>MFIKAERLLIRKFEFKDWEAVHEYTSDSDVMKYIPEGVFTEEDTRNFVNKNMGENAKNFPVILIGENILVGHIVFHKYFGEHTYEIGWVFNPKYFNKGYASEAAQATLKYGFKEMKLHRIIATCQPE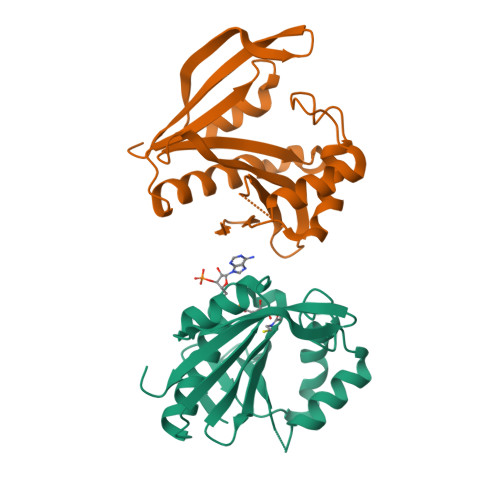NTPSYRVMEKIGMRREGYFKKCIPHGNEWWDEYYYAILEEE[2x]>[2x]DSVYVQNPQIPILVDRTDNVLFRIRIPDATKGDVLNRLTIRFGNEDKLSEVKAVRLFYAGTEAATKGRSRFAPVTYVSSHNIRNTRSANPSYSIRQDEVTTVANTLTLKTRQPMVKGINYFWVSVEMDRNTSLLSKLTSTVTEVVINDKPAVIAGEQAAVRRMGIGVRHAGDDGSASFRIPGLVTTNKGTLLGVYDVRYNN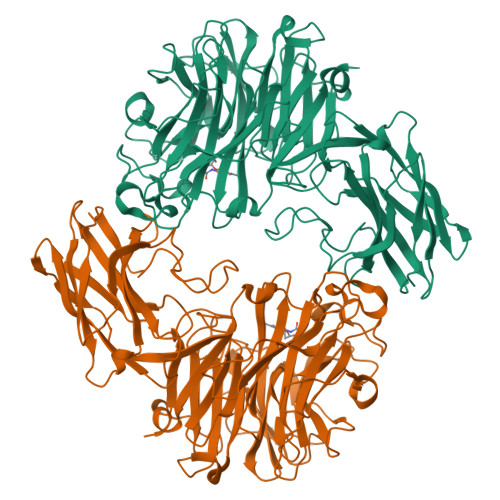SVDLQEHIDVGLSRSTDKGQTWEPMRIAMSFGETDGLPSGQNGVGDPSILVDERTNTVWVVAAWTHGMGNARAWTNSMPGMTPDETAQLMMVKSTDDGRTWSESTNITSQVKDPSWCFLLQGPGRGITMRDGTLVFPIQFIDSLRVPHAGIMYSKDRGETWHIHQPARTNTTEAQVAEVEPGVLMLNMRDNRGGSRAVSITRDLGKSWTEHSSNRSALPESICMASLISVKAKDNIIGKDLLLFSNPNTTEGRHHITIKASLDGGVTWLPAHQVLLDEEDGWGYSCLSMIDRETVGIFYESSVAHMTFQAVKIKDLIR> PSFDCGKPQVEPKKCPGRVVGGCVAHPHSWPWQVSLRTRFGMHFCGGTLISPEWVLTAAHCLEKSPRPSSYKVILGAHQEVNLEPHVQEIEVSRLFLEPTRKDIALLKLSSPAVITDKVIPACLPSPNYVVADRTECFITGWGETQGTFGAGLLKEAQLPVIENKVCNRYEFLNGRVQSTELCAGHLAGGTDSCQGDAGGPLVCFEKDKYILQGVTSWGL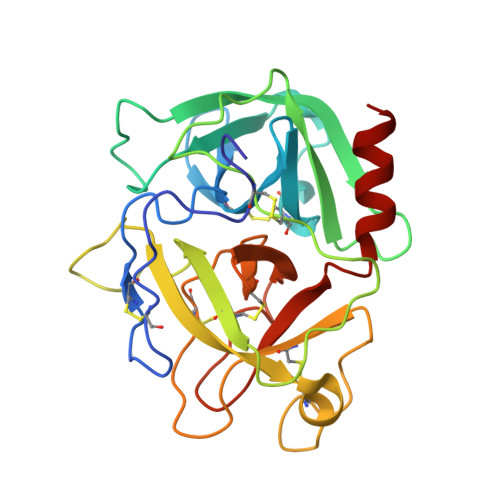GCARPNKPGVYVRVSRFVTWIEGVMRNN> SKLVMIFASMS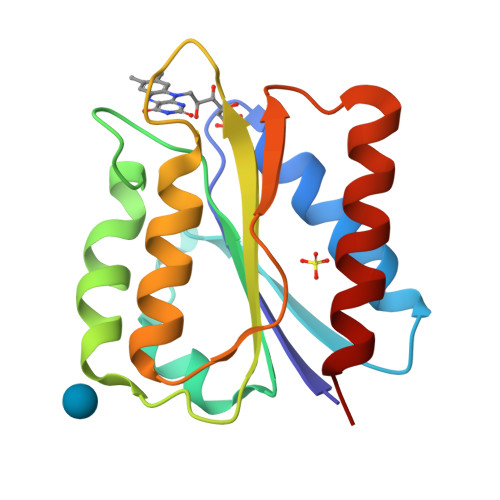GNTEEMADHIAGVIRETENEIEVIDIMDSPEASILEQYDGIILGAYTWGDGDLPDDFLDFYDAMDSIDLTGKKAAVFGSCDSAYPKYGVAVDILIEKLQERGAAVVLEGLKVELTPEDEDVEKCLQFGAEFVKHLS> MQNVKGGYWFKDSGLALNNIDSTLFTHLFCAFADLNPQLNQLIISPENQDSFRQFTSTVQRKNPSVKTFLSIAGGRANSTAYGIMARQPNSRKSFIDSSIRLARQLGFHGLDLDWEYPLSAADMTNLGTLLNEWRTAINTEARNSGRAALLLTAAVSNSPRVNGLNYPVESLARNLDWINLMAYDFYGPNWS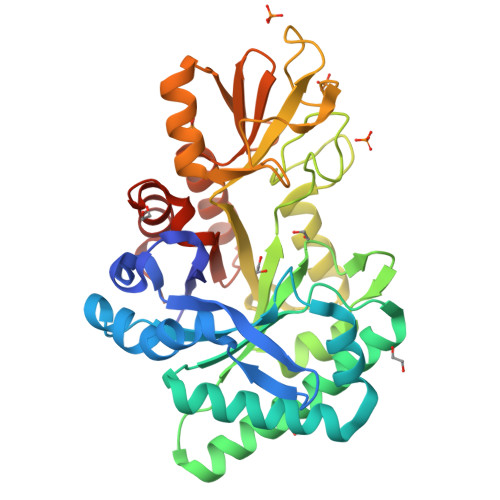PSQTNSHAQLFDPVNHVSGSDGINAWIQAGVPTKKLVLGIPFYGYAWRLVNANIHGLRAPAAGKSNVGAVDDGSMTYNRIRDYIVESRATTVYNATIVGDYCYSGSNWISYDDTQTVRNKVNYVKGRGLLGYFAWHVAGDQNWGLSRTASQTWGVSFQEMK> SNASEVKGKAPLELASGSAMVVDLQTNKVIYANNADEVVPIASITKLMTAMVVLDAKLPLDEIISVDIHQTKEMKGVFSRVRVNSEISRKDMLLLALMSSENRAAASLAHHYPGGYNAFINAMNAKAKSLGMTKTRYVEPTGLSINNVSTARDLTKLLIATKQYPLIGQLSTTTEKMATFREPNYTLPFRNTNHLVYNDKWNIQLTKTGFTNQ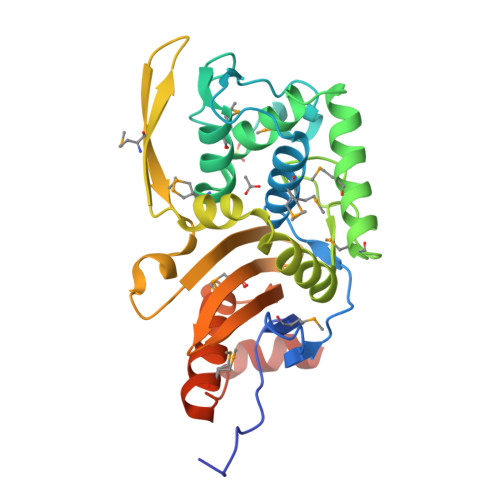AGHCLAMRTVIGNRPVALVVLDAFGKYTHFADANRLRSWMETGKAAPIPGAAKSYRQQKDAQGRLAQVSE>[2x]AEFKHVFVCVQDRPPGHPQGSCAQRGSREVFQAFMEKIQTDPQLFMTTVITPTGSMN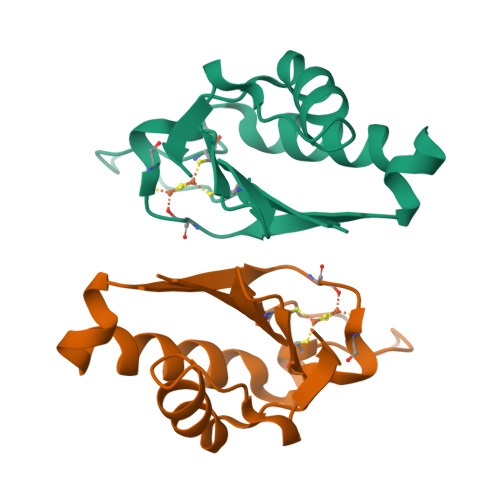ACMMGPVVVVYPDGVWYGQVKPEDVDEIVEKHLKGGEPVERLVISKGKPPGMF>[4x]MKGFAMLSIGKVGWIEKEKPAPGPFDAIVRPLAVAPCTSDIHTVFEGAIGERHNMILGHEAVGEVVEVGSEVKDFKPGDRVVVPAATPDWRTSEVQRGYHQHSGGMLAGWKFSNVKDGVFGEFFHVNDADMNLAHLPKEIPLEAAVMIPDMMTTGFHGAELA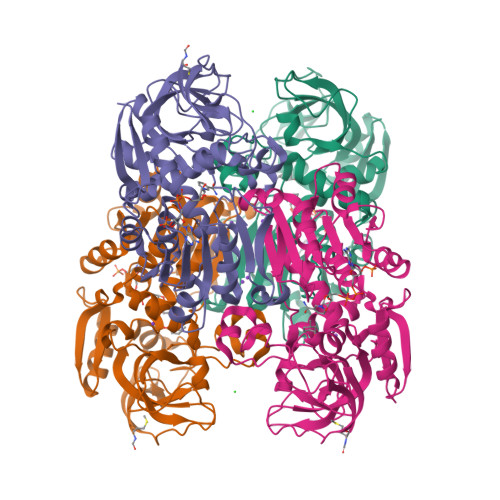DIELGATVAVLGIGPVGLMAVAGAKLRGAGRIIAVGSRPVCVDAAKYYGATDIVNYKDGPIESQIMNLTEGKGVDAAIIAGGNADIMATAVKIVKPGGTIANVNYFGEGEVLPVPRLEWGCGMAHKTIKGGLCPGGRLRMERLIDLVFYKRVDPSKLVTHVFRGFDNIEKAFMLMKDKPKDLIKPVVILA>[8x]SDTECHFCKSVINQAWNTSEQAMPQAMHQACLRFW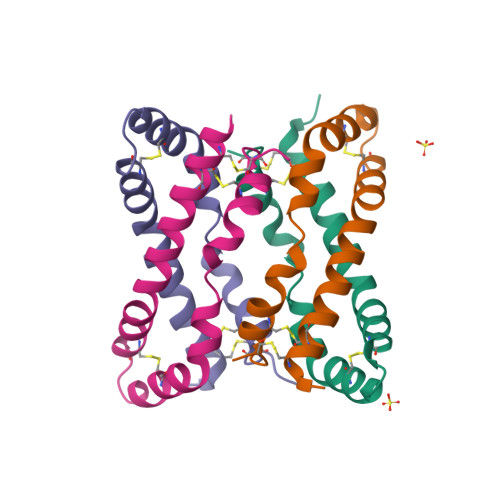LDRQKCEQFVEQHMPQLLALVPRSQDAHITCQALGVCEAPAS>[2x]MVGYSSKLIFVSMITRNGDRAPFANIENANYSWGTELSELTPIGMNQEYNLGLQLRKRYIDKFGLLPEHYVDQSIYVLSSHTNRTVVSAQSLLMGLYPAGTGPLIGDGDPAIKDRFQPIPIMTLSADSRLIQFPYEQYLAVLKKYVYNSPEWQNKTKEAAPNFAKWQQILGNRISGLNDVITVGDVLIVAQAHGKPLPKGLSQEDADQIIALTDWGLAQQFKS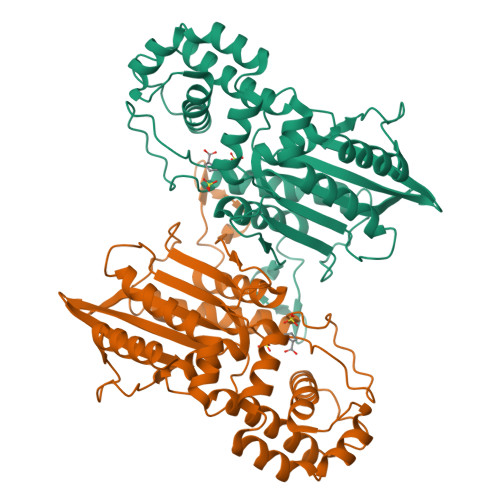QKVSYIMGGKLTNRMIEDLNNAVNGKSKYKMTYYSGHALTLLEVMGTLGVPLDTAPGYASNLEMELYKDGDIYTVKLRYNGKYVKLPIMDKNNSCSLDALNKYMQSINEKFQKHHHHHH>[2x]GAMGYDYDYLFKIVLIGDSGVGKSNLLSRFTTDEFNIESKSTIGVEFATRTIEVENKKIKAQIWDTAGLERYRAITSAYYRGAVGALIVYDISKSSSYENCNHWL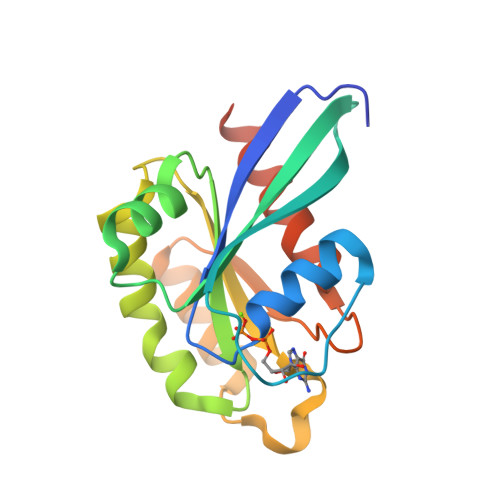TELRENADDNVAVGLIGNKSDLAHLRAVPTDEAKNFAMENQMLFTETSALNSDNVDKAFRELIVAIFQMVSKHQVDLSGS>[18x]SMLDRELESSAPGVPSVSVHPLLGSHVVLPQEPEEHLWQGDVGTEAHPWLSDHRVHQVAVLPGAAYCEMALAAVTPVLGDTGEVHDLKFHDMLLLDDATPVWVSAAVTAPGTAEFGVETHQSGDRTQRATAVLRGDVDAERPAAHSIDALLAAHPNRVDGDELRAGFGTVGIGHGAAFAGLSEAYVATAAEPTVVAAVALPGPLRSGQRGYTVHPALLDACFQSVIAHPEVQNIASGMLLPLGVRRLRAYGSTRNVRYCLSRIVKADSFGVEADLELLDADGTVLLSAMGLQLGTGNSDKAEEERLLDERLLTIEWQQRELPRPEGSETVDAGSWLVILAGDDDENPRAAGVVSALIGAGMPTTTMAWSHDADHDAQAAALTARLDEQPLAGVAVIVGDSETGTDAHDVGADARRGADHVRHLVRIARTLADAVGEPPRLYVVTHRSQHVLDTDEPYLEHSGLRGLIRVVGMEHPRLRATQIDVDDSTAHEALVRQLLSGSPEDETAWRDGQWYAARLCPSPLRAAERRTAVADNASEGMRLVVRNPGDLESMELVTFERGTPGPGQIEVAVKASSINFADVLVAFGR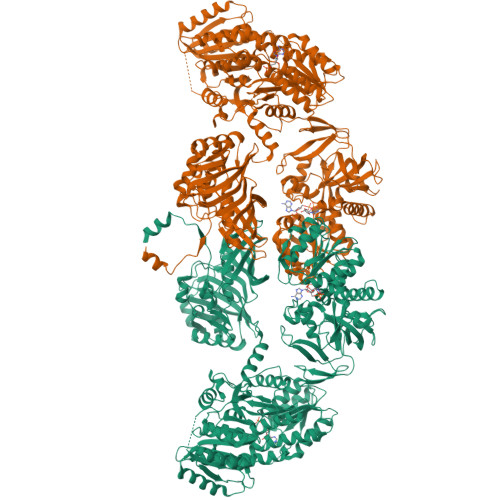CPSFDGRLPELGSEFGGVVTAVGPGVTTHRVGDRVGGVSANGCWSNFVTCEADLATKLPEGISEHEAAAVGLAYGTVWLGLTELARMSAGDKILIHSATGGVGQAAIAVARAAGAEIYATAGSEKRRQLLRDWGIEHVYDSRTTAFADQIRTDTDGYGVDIVLNSVTGPAQRAGLELLAFGGRFVEIGKRDIYADTRLGLFPFRRNLSFYAVDLALMTVTHPQKIRDLLATVYRLIADGTLPLPEITHYPLEEAATAIRIMGGAQHTGKLVIDIPDTGQSQVVVPPEQVPVFRGDGAYVITGGLGGLGLFLAERMAAAGCGRIVVNSRSAPSTRSSEIIELIRATGADIVVECGDIAEPDTALRLVAAATQTGLPLRGVLHAAAVVEDATLANITDELVEHDWAPKVYGAWNLHQAVQSGGPATSELDWFCAFSSAAALVGSPGQGAYAAANSWLDAFMQWRRAQGLPATSIAWGAWGEIGRGTAMAEGDNAIAPDEGAYAFEAILRHDRVYNGYAPVLGASWLTAFAQRSPFAELFLADTQGASETRKLRQ5-[[3,5-bis(chloranyl)phenyl]sulfonylamino]-2-[(5-bromanyl-4-fluoranyl-2-methyl-phenyl)sulfamoyl]benzoic 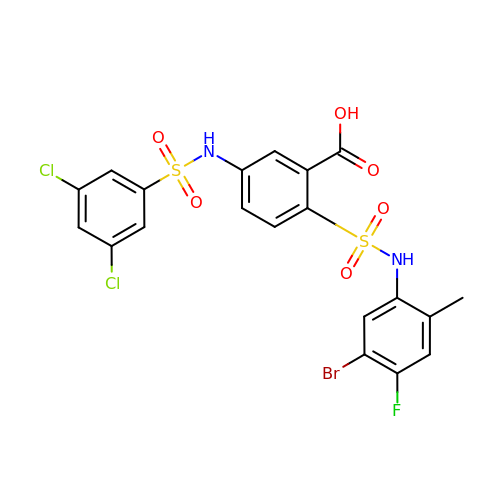acid | C20 H14 Br Cl2 F N2 O6 S2 | MJYYUGUIBHEWRX-UHFFFAOYSA-N1,5-BIS(N-BENZYLOXYCARBONYL-L-LEUCINYL)CARBOHYDRAZIDE | C29 H40 N6 O7 | 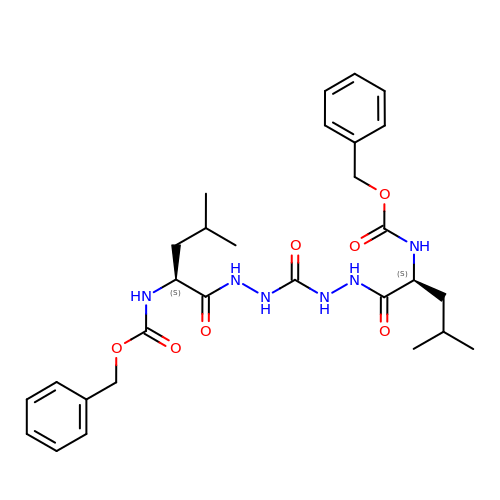HGDUWJVGIGLVOH-ZEQRLZLVSA-N> MAAQVTLEDALSNVDLLEELPLPDQQPCIEPPPSSLLYQPNFNTNFEDRNAFVTGIARYIEQATVHSSMNEMLEEGQEYAVMLYTWRSCSRAIPQVKCNEQPNRVEIYEKTVEVLEPEVTKLMNFMYFQRNAIERFCGEVRRLCHAERRKDFVSEAYLITLGKFINMFAVLDELKNMKCSVKNDHSAYKRAAQFLRKMADPQSIQESQNLSMFLANHNKITQSLQQQLEVISGYEELLADIVNLCVDYYENRMYLTPSEKHMLLKVMGFGLYLMDGSVSNIYKLDAKKRINLSKIDKYFKQLQVVPLFGDMQIELARYIKTSAHYEENKSRWTCTSSGSSPQYNICEQMIQIREDHMRFISELARYSNSEVVTGSGRQEAQKTDAEYRKLFDLALQGLQLLSQWSAHVMEVYSWKLVHPTDKYSNKDCPDSAEEYERATRYNYTSEEKFALVEVIAMIKGLQVLMGRMESVFNHAIRHTVYAALQDFSQVTLREPLRQAIKKKKNVIQSVLQAIRKTVCDWETGHEPFNDPALRGEKDPKSGFDIKVPRRAVGPSSTQLYMVRTMLESLIADKSGSKKTLRSSLEGPTILDIEKFHRESFFYTHLINFSETLQQCCDLSQLWFREFFLELTMGRRIQFPIEMSMPWILTDHILETKEASMMEYVLYSLDLYNDSAHYALTRFNKQFLYDEIEAEVNLCFDQFVYKLADQIFAYYKVMAGSLLLDKRLRSECKNQGATIHLPPSNRYETLLKQRHVQLLGRSIDLNRLITQRVSAAMYKSLELAIGRFESEDLTSIVELDGLLEINRMTHKLLSRYLTLDGFDAMFREANHNVSAPYGRITLHVFWELNYDFLPNYCYNGSTNRFVRTVLPFSQEFQRDKQPNAQPQYLHGSKALNLAYSSIYGSYRNFVGPPHFQVICRLLGYQGIAVVMEELLKVV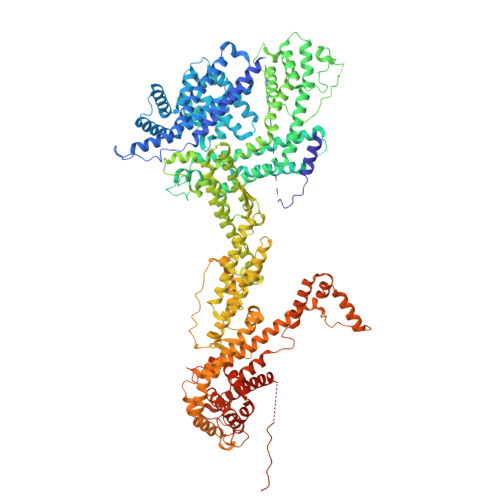KSLLQGTILQYVKTLMEVMPKICRLPRHEYGSPGILEFFHHQLKDIVEYAELKTVCFQNLREVGNAILFCLLIEQSLSLEEVCDLLHAAPFQNILPRVHVKEGERLDAKMKRLESKYAPLHLVPLIERLGTPQQIAIAREGDLLTKERLCCGLSMFEVILTRIRSFLDDPIWRGPLPSNGVMHVDECVEFHRLWSAMQFVYCIPVGTHEFTVEQCFGDGLHWAGCMIIVLLGQQRRFAVLDFCYHLLKVQKHDGKDEIIKNVPLKKMVERIRKFQILNDEIITILDKYLKSGDGEGTPVEHVRCFQPPIHQSLASS> GPLGSNYNQLKEDYNTLKRELSDRDDEVKRLREDIAKENELRTKAEEEADKLNKEVEDLTA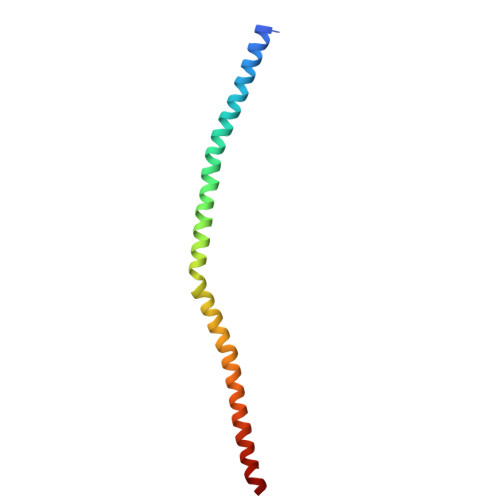SLFDEANNMVADARKEKYAIEILNKRLTEQLREKDT>[2x]MTYGIVIVSHSPEIASGLKKLIREVAKNISLTAIGGLENGEIGTSFDRVMNAIEENEADNLLTFFDLGSARMNLDLVSEMTDKELTIFNVPLIE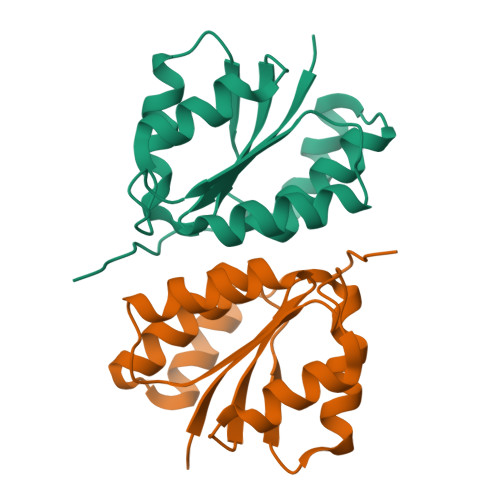GAYTASALLEAGATFEAIKEQLEKMLIEKRSHHHHHH>[9x]SDFVVIKALEDGVNVI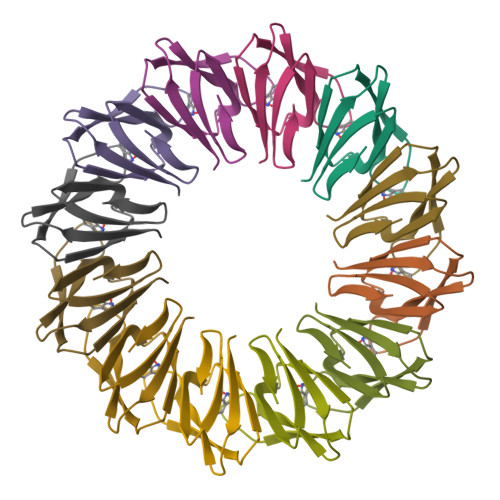GLTRGADTRFHHSEKLDKGEVLIAQFTEHTSAIKVRGKAYIQTRHGVIE>[4x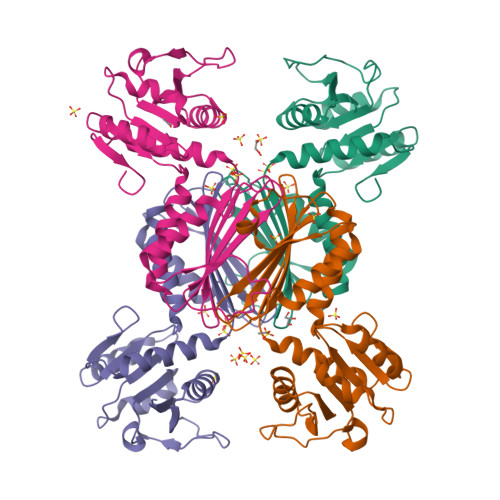]MASMKILLIGYGAMNQRVARLAEEKGHEIVGVIENTPKATTPYQQYQHIADVKGADVAIDFSNPNLLFPLLDEDFHLPLVVATTGEKEKLLNKLDELSQNMPVFFSANMSYGVHALTKILAAAVPLLDDFDIELTEAHHNKKVDAPSGTLEKLYDVIVSLKENVTPVYDRHELNEKRQPQDIGIHSIRGGTIVGEHEVLFAGTDETIQITHRAQSKDIFANGAIQAAERLVNKPNGFYTFDNL> AGRR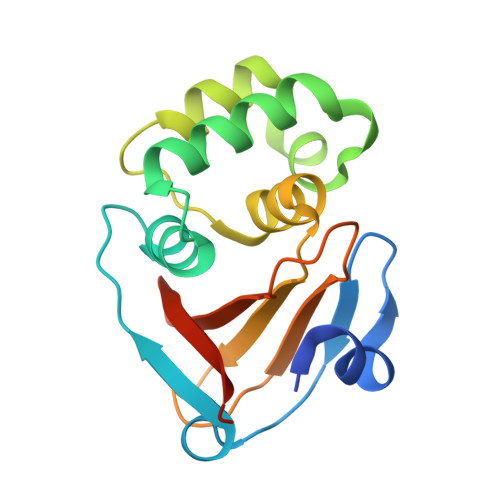RSSNLSESLISDCDNLGNFYRGPIVLDINKEFTIEDVPGDGDCFFHCLAKQLPEVSVSRLKGIITSYALRNWDTLTEAPRFYSDPKDYERELNRAGYWGGTTEAEIINHSFGVPVVIWTTEDKKLTSAVQVWTRKHGNLPELHLLHTGTHFMCLAPIVKEGTPPRE>MSLTKIPENVQGAVS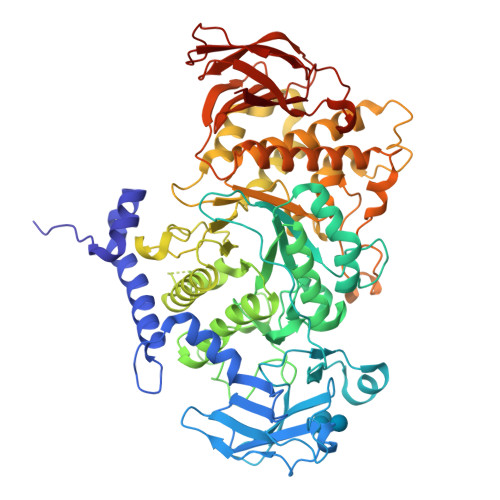IDPWLEPFADVLSERRYLADKWLYDIKHATPDGSEQSLVDFARNAYKTYGLHANQQTKEIVYREWAPNAQRAFLVGEFNNWNEESHEMKHKDEFGVFSITLAPLENGDFAIPHDSKIKVMFVLPDGSKVYRIPAWITRATQPSKETAQKYGPTYEGRFWNPPNSYQFKHQRPKFNLANDSIKIYEAHIGISSPEPKVASYKEFTQNVLPRIKHLGYDAIQLMAIMEHAYYASFGYQVTNFFAISSRYGTPEDLKELIDTAHSMGILVLLDVIHSHASKNSEDGLNMFDGSDHQYFHSLTSGRGEHPLWDSRLFNYGSFEVQRFLLANLAYYIDVYQFDGFRFDGVTSMLYLHHGVGAGGAFSGDYNEYLSRDRSGVDHEALAYLMLANDLVHDLLPESAVTIAEDVSGYPTLCLPRTAGGGGFDYRLAMALPDMWIKLLKTKQDDDWDMGHIVHTLTNRRHGEKVVAYCESHDQALVGDKTLAFWLMDAAMYTDMTVLKEPTLVIDRGIALHKMIRLITHSLGGEAYLNFEGNEFGHPEWLDFPRVGNNDSYHYARRQFNLVDDDLLRYRHLNEFDAAMQNCESKHQWLNTPQAYVSLKHEVDKVIAFERNGHLFVFNFHPTQSFTDYRIGVDVAGTYKIVLNTDRAEFGGHNRIDEAQEFFTTDLEWNNRRNFIQVYIPSRTAIVLTRQM[2x]> MQRARCYLIGETAVVLELEPPVTLASQKRIWRLAQRLVDMPNVVEAIPGMNNITVILRNPESLALDAI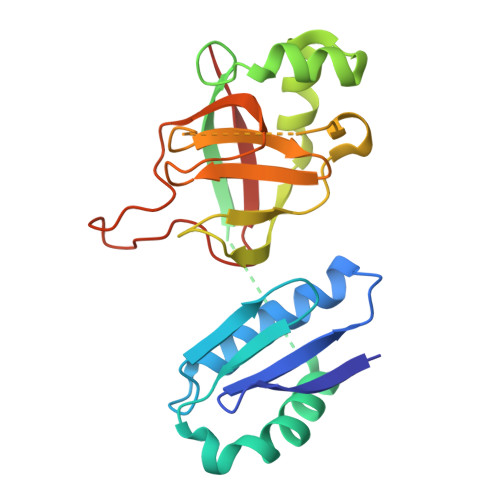ERLQRWWEESEALEPESRFIEIPVVYGGAGGPDLAVVAAHCGLSEKQVVELHSSVEYVVWFLGFQPGFPYLGSLPEQLHTPRRAEPRLLVPAGSVGIGGPQTGVYPLATPGGWQLIGHTSLSLFDPARDEPILLRPGDSVRFVPQKEGVC> SVTLRDLFDRAVVLSHYIHNLSSEMFSEFDKRYTHGRGFITKAINSCHTSSLATPEDKEQAQQMNQKDFLSLIVSILRSWNEPLYHLVTEVRGMQEAPEAILSKAVEIEEQTKRLLERMELIVSQVHPETKENEIYPVWSGLPSLQMADEESRLSAYYNLLHC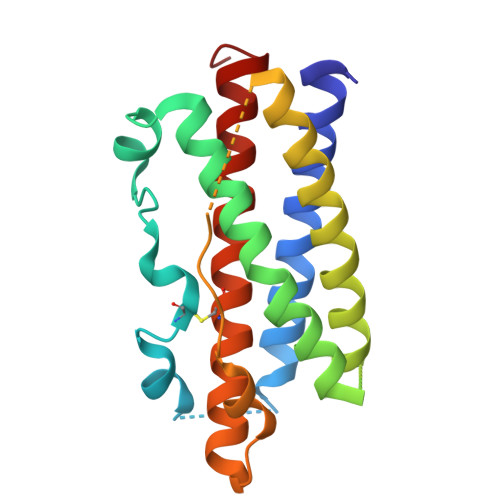LRRDSHKIDNYLKLLKCRIIHNNNC> GMAANGGDHTSARPHVVLLPSAGMGHLVPFARLAVALSEGHGCNVSVAAVQPTVSSAESRLLDALFVAAAPAVRRLDFRLAPFDESEFPGADPFFLRFEATRRSAP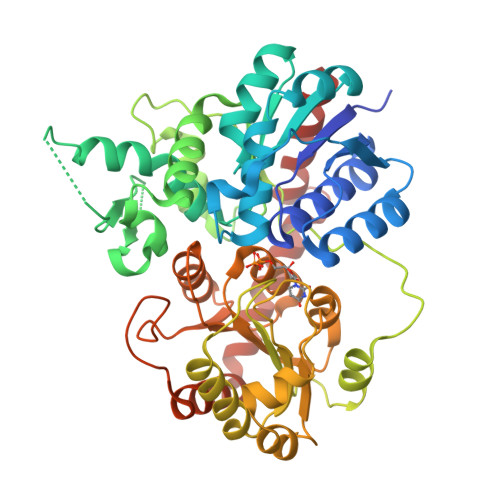LLGPLLDAAEASALVTDIVLASVALPVARERGVPCYVLFTSSAAMLSLCAYFPAYLDAHAAAGSVGVGVGNVDIPGVFRIPKSSVPQALHDPDHLFTQQFVANGRCLVACDGILVNTFDAFEPDAVTALRQGSITVSGGFPPVFTVGPMLPVRFQAEETADYMRWLSAQPPRSVVYVSFGSRKAIPRDQLRELAAGLEASGKRFLWVVKSTIVDRDDTADLGGLLGDGFLERVQGRAFVTMGWVEQEEILQHGSVGLFISHCGWNSLTEAAAFGVPVLAWPRFGDQRVNAALVARSGLGAWEEGWTWDGEEGLTTRKEVAKKIKGMMGYDAVAEKAAKVGDAAAAAIAKCGTSYQSLEEFVQRCRDAERK(7aR,8R)-8-amino-4-cyclopropyl-12-fluoro-1-oxo-4,7,7a,8,9,10-hexahydro-1H-pyrrolo[1',2':1,7]azepino[2,3-h]quinoline-2-carboxylic 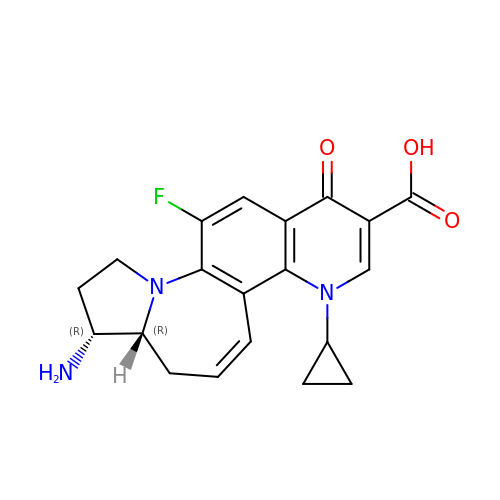acid | C20 H20 F N3 O3 | KZNQXATUOHSRHR-HZPDHXFCSA-N>[6x]SG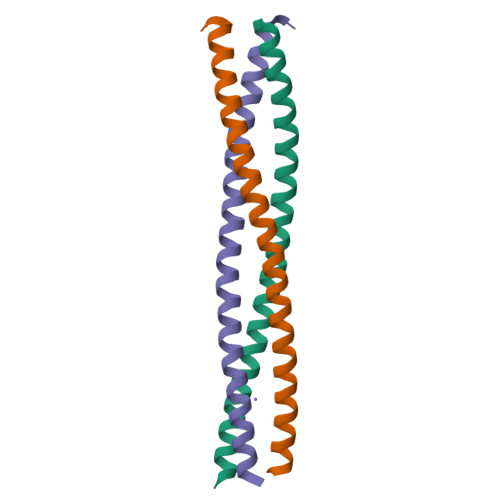SVEDRVTQLERISNAHSQLLTQLQQQLSDNQSDIDSLRGQIQENQYQLNQVVERQKQILLQIDSLSSGGAAAQLEHHHHHH> MNVYDDVLDATVVSHSLATHFTTSDYEELLVVRTNILSVYRPTRDGKLYLTDEFKFHGLITDIGLIPQKDSPLSCLLLCTGVAKISILKFNTLTNSIDTLSLHYYEGKFKGKSLVELAKISTLRMDPGSSCALLFNNDIIAFLPFHVNKNDDDEEEEDEDENIDDSELIHSMNQKSQGTNTFNKRKRTKLGDKFTAPSVVLVASELYEGAKNIIDIQFLKNFTKPTIALLYQPKLVWAGNTTISKLPTQYVILTLNIQPAESATKIESTTIAFVKELPWDLHTIVPVSNGAIIVGTNELAFLDNTGVLQSTVLLNSFADKELQKTKIINNSSLEIMFREKNTTSIWIPSSKSKNGGSNNDETLLLMDLKSNIYYIQMEAEGRLLIKFDIFKLPIVNDLLKENSNPKCITRLNATNSNKNMDLFIGFGSGNALVLRLNNLKSTIETREAHNPSSGTNSLMDINDDDDEEMDDLYADEAPENGLTTNDSKGTVETVQPFDIELLSSLR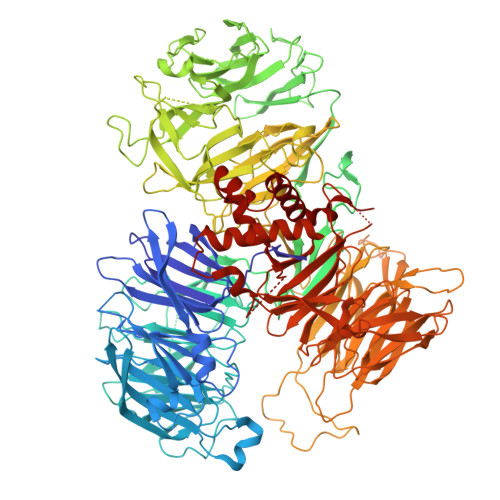NVGPITSLTVGKVSSIDDVVKGLPNPNKNEYSLVATSGNGSGSHLTVIQTSVQPEIELALKFISITQIWNLKIKGRDRYLITTDSTKSRSDIYESDNNFKLHKGGRLRRDATTVYISMFGEEKRIIQVTTNHLYLYDTHFRRLTTIKFDYEVIHVSVMDPYILVTVSRGDIKIFELEEKNKRKLLKVDLPEILNEMVITSGLILKSNMCNEFLIGLSKSQEEQLLFTFVTADNQIIFFTKDHNDRIFQLNGVDQLNESLYISTYQLGDEIVPDPSIKQVMINKLGHDNKEEYLTILTFGGEIYQYRKLPQRRSRFYRNVTRNDLAITGAPDNAYAKGVSSIERIMHYFPDYNGYSVIFVTGSVPYILIKEDDSTPKIFKFGNIPLVSVTPWSERSVMCVDDIKNARVYTLTTDNMYYGNKLPLKQIKISNVLDDYKTLQKLVYHERAQLFLVSYCKRVPYEALGEDGEKVIGYDENVPHAEGFQSGILLINPKSWKVIDKIDFPKNSVVNEMRSSMIQINSKTKRKREYIIAGVANATTEDTPPTGAFHIYDVIEVVPEPGKPDTNYKLKEIFQEEVSGTVSTVCEVSGRFMISQSQKVLVRDIQEDNSVIPVAFLDIPVFVTDSKSFGNLLIIGDAMQGFQFIGFDAEPYRMISLGRSMSKFQTMSLEFLVNGGDMYFAATDADRNVHVLKYAPDEPNSLSGQRLVHCSSFTLHSTNSCMMLLPRNEEFGSPQVPSFQNVGGQVDGSVFKIVPLSEEKYRRLYVIQQQIIDRELQLGGLNPRMERLANDFYQMGHSMRPMLDFNVIRRFCGLAIDRRKSIAQKAGRHAHFEAWRDIINIEFSMRSLCQGK trans-Ned 19 | C30 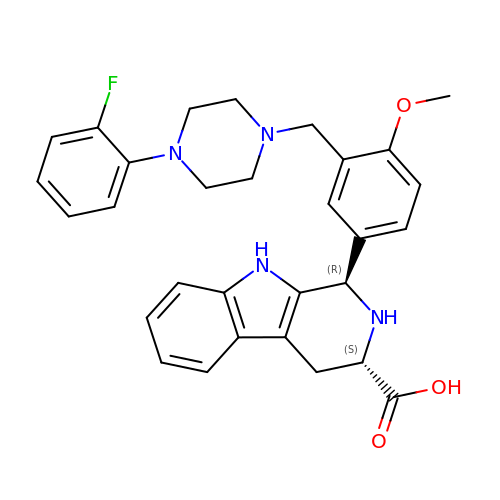H31 F N4 O3 | FUHCEERDBRGPQZ-LBNVMWSVSA-N> SSNTRVALVTGANKGIGFAIVRDLCRQFAGDVVLTARDVARGQAAVKQLQAEGLSPRFHQLDIIDLQSIRALCDFLRKEYGGLDVLVNNAAIAFQLDNPTPFHIQAELTMKTNFMG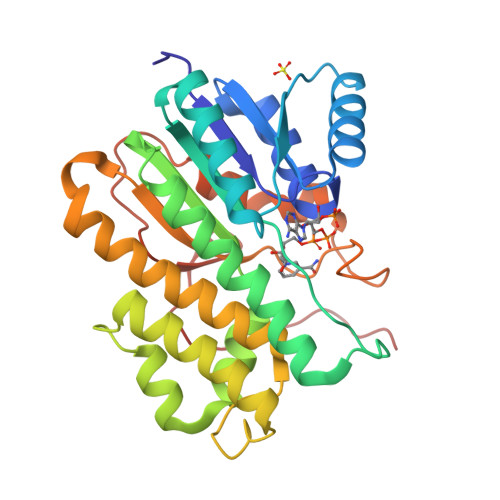TRNVCTELLPLIKPQGRVVNVSSTEGVRALNECSPELQQKFKSETITEEELVGLMNKFVEDTKNGVHRKEGWSDSTYGVTKIGVSVLSRIYARKLREQRAGDKILLNACCPGWVRTDMGGPKAPKSPEVGAETPVYLALLPSDAEGPHGQFVTDKKVVEWGVPPESYPWVNA> GPGSEFQECAVCGWALPHNRMQALTSCECTICPDCFRQHFTI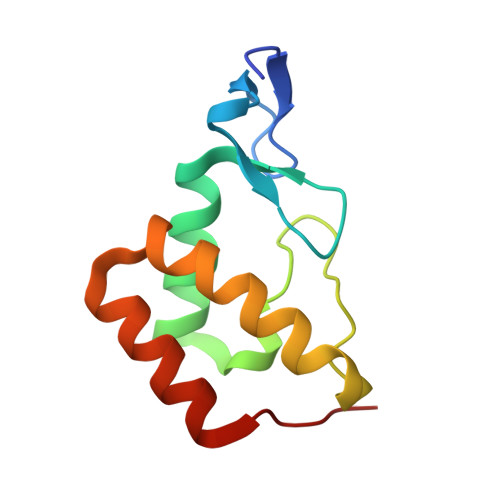ALKEKHITDMVCPACGRPDLTDDTQLLSYFSTLDIQLRESLEPDAYALFHKKLTEGVLMRD> GGGNHQHI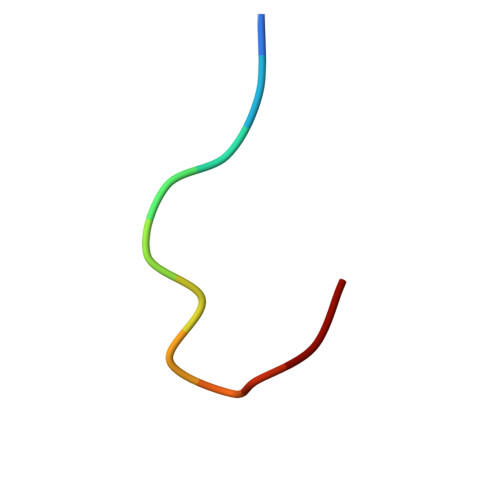GKP> MPYIEKLELKGFKSYGNKKVVIPFSKGFTAIVGANGSGKSNIGDAILFVLGGLSAKAMRASRISDLIFAGSKNEPPAKYAEVAIYFNNEDRGFPIDEDEVVIRRRVYPDGRSSYWLNGRRATRSEILDILTAAMISPDGYNIVLQGDITKFIKMSPLERRLLIDDISGIAEYDSKKEKALEELKQAEENLARVDLLIKEVKSGGSGGSDFEIVERRYLELKSKREKLEAEKESIIEFINEIEKEKKNVFMRTFEAISRNFSEIFAKLSPGGSARLILENPEDPFSGGLEIEAKPAGKDVKRIEAMSGGEKALTALAFVFAIQKFKPAPFYLFDEIDAHLDDANVKRVADLIKESSKESQFIVITLRDVMMANADKIIGVSMRDGVSKVVSLSLEKAMKILEEIRK;> DIEKYVEELYKVVKKIYEKTGTPIKFWDLVPDVEPKIIARTFLYLLFLENMGRVEIIQEEPFGEILVVPMVDKL

Multi-subunit SMC complexes control chromosome superstructure and promote chromosome disjunction, conceivably by actively translocating along DNA double helices. SMC subunits comprise an ABC ATPase “head” and a “hinge” dimerization domain connected by a 49 nm coiled-coil “arm. The heads undergo ATP-dependent engagement and disengagement to drive SMC action on the chromosome. Here, we elucidate the architecture of prokaryotic Smc dimers by high-throughput cysteine cross-linking and crystallography.

We noticed that all residues on the Smc head domain, which were cross-linked by BMOE when substituted for cysteine, map to a relatively small surface area.Dyclonine | C18 H27 N O2 | 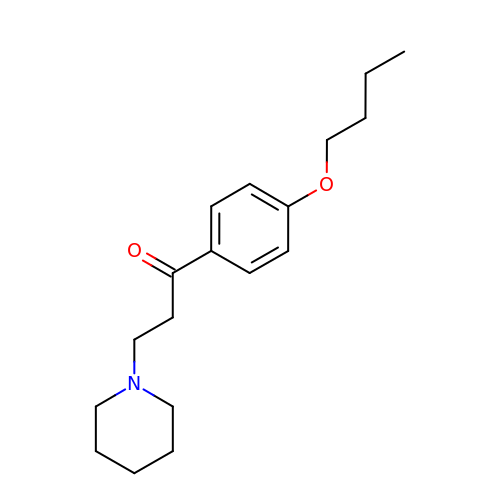BZEWSEKUUPWQDQ-UHFFFAOYSA-N> RSMAAEVYFGDLELFEPFDHPGESIPKPVHTRFKDDDGDEEDENGVGDAELRERLRQCEETIEQLRAENQELKRKLNILTRPSGILVNDTKLDGPILQILFMNNAISKQYHQEIEEFVSNLVKRFEEQQKNDVEKTSFNLLPQPSSIVLEEDHKVEESCAIKNNKEAFSVVGSVLYFTNFCLDKLGQPLLNENPQLSEGWEIPKYHQVFSHIVSLEGQEIQVKAKRPKPHCFNCGSEEHQMKDCPMPRNAARISEKRKEYMDACGEANNQNFQQRYHAEEVEERFGRFKPGVISEELQDALGVTDKSLPPFIYRMRQLGYPPGWLKEAELENSGLALYDGKDGTDGETEVGEIQQNKSVTYDLSKLVNYPGFNISTPRGIPDEWRIFGSIPMQACQQKDVFANYLTSNFQAPGVKSGNKRSSSHSSPGSPKKQKNESNSAGSPADMELDSDMEVPHGSQSSESFQFQPPLPPDTPPLPRGTPPPVFTPPLPKGTPPLTPSDSPQTRTGSGAVDEDALTLEELEEQQRRIWAALEQAESVNSDSDVPVDTPLTGNSVASSPCPNELDLPVPEGKTSEKQTLDEPEVPEIFTKKSEAGHASSPDSEVTSLCQKEKAELAPVNTEGALLDNGSVVPNCDISNGGSQKLFPADTSPSTATKIHSPIPDMSKFATGITPFEFENMAESTGMYLRIRSLLKNSPRNQQKNKKASE;> GPDSMADAFGDELFSVFEGDSTTAAGTKKDKEKDKGKWKGPPGSADKAGKRFDGKLQSESTNNGKNKRDVDFEGTDEPIFGKKPRIEESITEDLSLADLMPRVKVQSVETVEGCTHEVALPAEEDYLPLKPRVGKAAKEYPFILDAFQREAIQCVDNNQSVLVSAHTSAGKTVCAEYAIALALREKQRVIFTSPIKALSNQKYREMYEEFQDVGLMTGDVTINPTASCLVMTTEILRSMLYRGSEVMREVAWVIFDEIHYMRDSERGVVWEETIILLPDNVHYVFLSATIPNARQFAEWICHLHKQPCHVIYTDYRPTPLQHYIFPAGGDGLHLVVDENGDFREDNFNTAMQVLRDAGDLAKGDQKGRKGGTKGPSNVFKIVKMIMERNFQPVIIFSFSKKDCEAYALQMTKLDFNTDEEKKMVEEVFSNAIDCLSDEDKKLPQVEHVLPLLKRGIGIHHGGLLPILKETIEILFSEGLIKALFATETFAMGINMPARTVLFTNARKFDGKDFRWISSGEYIQMSGRAGRRGMDDRGIVILMVDEKMSPTIGKQLLKGSADPLNSAFHLTYNMVLNLLRVEEINPEYMLEKSFYQFQHYRAIPGVVEKVKNSEEQYNKIVIPNEESVVIYYKIRQQLAKLGKEIEEYIHKPKYCLPFLQPGRLVKVKNEGDDFGWGVVVNFSKKSNVKPNSGELDPLYVVEVLLRCSKESLKNSATEAAKPAKPDEKGEMQVVPVLVHLLSAISSVRLYIPKDLRPVDNRQSVLKSIQEVQKRFPDGIPLLDPIDDMGIQDQGLKKVIQKVEAFEHRMYSHPLHNDPNLETVYTLCEKKAQIAIDIKSAKRELKKARTVLQMDELKCRKRVLRRLGFATSSDVIEMKGRVACEISSADELLLTEMMFNGLFNDLSAEQATALLSCFVFQENSSEMPKLTEQLAGPLRQMQECAKRIAKVSAEAKLEIDEETYLSSFKPHLMDVVYTWATGATFAHICKMTDVFEGSIIRCMRRLEELLRQMCQAAKAIGNTELENKFAEGITKIKRDIVFAASLYL

The nuclear exosome targeting (NEXT) complex plays a central role in directing non-functional transcripts to exosome-mediated degradation, but the structural and molecular mechanisms remain enigmatic. Here, we elucidated the architecture of the human NEXT complex, showing that it exists as a dimer of MTR4-ZCCHC8-RBM7 heterotrimers. Dimerization preconfigures the major MTR4-binding region of ZCCHC8 and arranges the two MTR4 helicases opposite to each other, with each protomer able to function on many types of RNAs. In terms of architecture, we found that the biological unit of NEXT consists of two copies of each MTR4 and RBM7, assembling symmetrically around a highly intertwined ZCCHC8 homodimer, with an arrangement conducive for targeting different RNA substrates.

The 7 Å resolution cryo-EM map of the NEXTL sample also revealed additional density features near and/or within the expected RNA-binding site of the DExH-box domain. To better resolve this portion of the complex, we focused the cryo-EM processing solely on the MTR4 DExH-box domain, allowing us to obtain a reconstruction with a local resolution of 3.4 Å. The resulting cryo-EM reconstruction, inspected at low map threshold, showed density at the bottom of the DExH-box domain consistent with the presence of the ZCCHC8 C-terminal domain (CTD, residues 659–700) as observed in the corresponding crystal structure. Briefly, the ZCCHC8 CTD binds along the bottom of the DExH-box domain, starting from RecA1 and ending at RecA2, in the proximity of AMPPNP. However, additional density was present inside the helicase channel of MTR4. The MTR4 helicase channel is known to bind RNA in a defined polarity, with the 5′ and 3′ ends near the top and bottom surfaces, respectively, of the DExH-box domain (Gerlach et al., 2018; Weick et al., 2018; Weir et al., 2010). Starting from the top surface of the DExH-box domain, the cryo-EM map showed well defined density for the first four nucleotides and less resolved density for the fifth one. The structural analysis suggested that the ZCCHC8 CTD encloses the RNA by gating the exit of the RNA channel—similar to a gatekeeping feature we recently identified in the cytoplasmic cofactor of the exosome (Kögel et al., 2022). Importantly, the addition of separately purified ZCCHC8 CTD in trans to both NEXTS and NEXTSmono recapitulated the compact footprint of NEXTL, supporting the notion that the ZCCHC8 CTD restricts benzonase access to RNA substrates by gating one side of the RNA-binding path. In the inactive state of the complex, the 3′ end of an RNA substrate is enclosed in the MTR4 helicase channel by a ZCCHC8 C-terminal gatekeeping domain.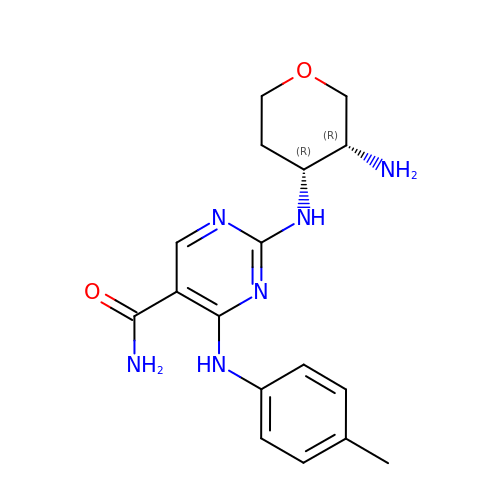2-{[(3R,4R)-3-aminotetrahydro-2H-pyran-4-yl]amino}-4-[(4-methylphenyl)amino]pyrimidine-5-carboxamide | C17 H22 N6 O2 | KBPYMFSSFLOJPH-UONOGXRCSA-N> SKSSSSRRNAWGNLSYADLITKAIESSAEKRLTLSQIYEWMVKSVPYFKDKGDSNSSAGWKNSIRHNLS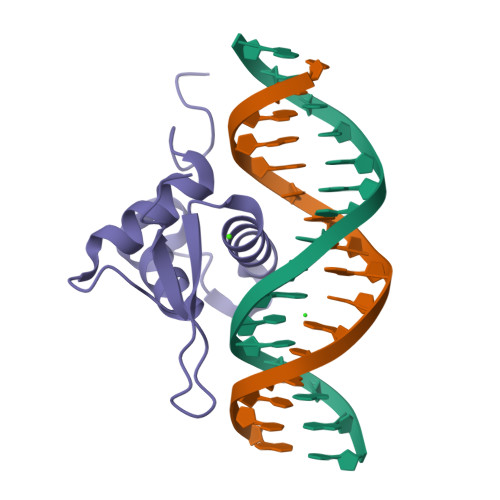LHSKFIRVQNEGTGKSSWWMLNPEGGKSGKS[[(2~{R},3~{S})-5-(6-aminopurin-9-yl)-4-oxidanyl-3-phosphonooxy-oxolan-2-yl]methoxy-oxidanyl-phosphoryl] 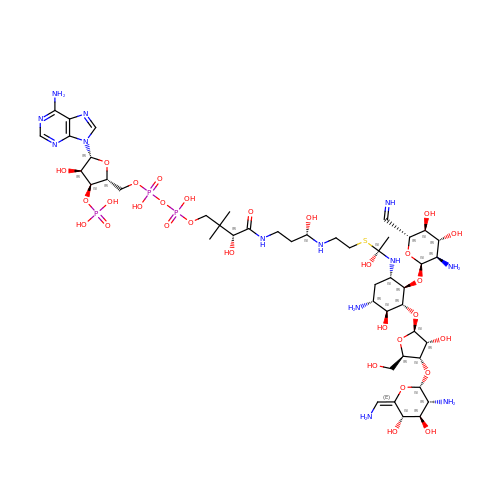[(3~{R})-4-[[(3~{S})-3-[2-[(1~{S})-1-[[(1~{S},2~{R},3~{R},4~{S},5~{R})-5-azanyl-3-[(4~{S},5~{R})-4-[(2~{S},3~{R},4~{R},5~{S},6~{E})-3-azanyl-6-(azanylmethylidene)-4,5-bis(oxidanyl)oxan-2-yl]oxy-5-(hydroxymethyl)-3-oxidanyl-oxolan-2-yl]oxy-2-[(2~{S},3~{R},4~{R},5~{S})-3-azanyl-6-(iminomethyl)-4,5-bis(oxidanyl)oxan-2-yl]oxy-4-oxidanyl-cyclohexyl]amino]-1-oxidanyl-ethyl]sulfanylethylamino]-3-oxidanyl-propyl]amino]-2,2-dimethyl-3-oxidanyl-4-oxidanylidene-butyl] hydrogen phosphate | C46 H82 N13 O30 P3 S | KNUGXPWVQDBKDV-VYRIPBRXSA-N>ILGGREAEAHARPYMASVQLNGAHLCGGVLVAEQWVLSAAHCLEDAADGKVQVLLGAHSLSQPEPSKRLYDVLRAVPHPDSQPDTIDHDLLLLQLSEKATLGPAVRPLPWQRVDRDVAPGTLCDVAGWGIVNHAGRRPDSLQHVLLPVLDRATCNRRTHHDGAITERLMCAESNRRDSCKGDSGGPLVCGGVLEG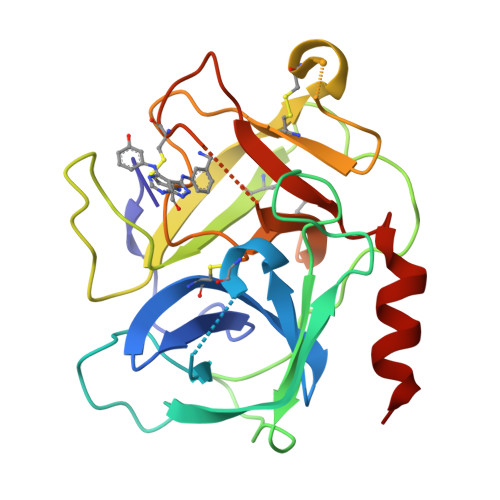VVTSGSRVCGNRKKPGIYTRVASYAAWIDSVLASAAA[6x]>[4x]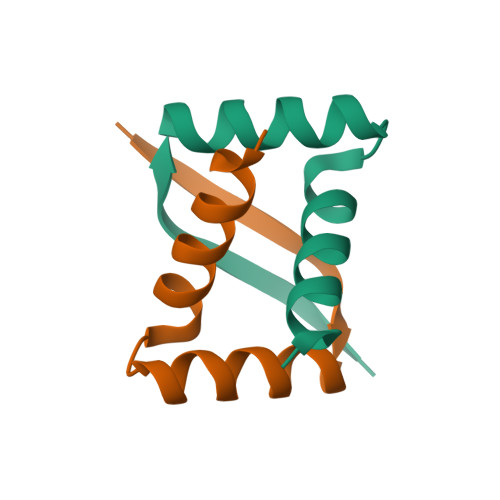MSAMVQIRNVPDELLHELKARAAAQRMSLSDFLLARLAEIAEEP> MDSTSTIANKIEEYLGAKSDDSKIDELLKADPSEVEYYRSGGDGDYLKNNICKITVNHSDSGKYDPCEKKLPPYDDNDQWKCQQNSSDGSGKPENICVPPRRERLCTYNLENLKFDKIRDNNAFLADVLLTARNEGEKIVQNHPDTNSSNVCNALERSFADLADIIRGTDQWKGTNSNLEKNLKQMFAKIRENDKVLQDKYPKDQKYTKLREAWWNANRQKVWEVITCGARSND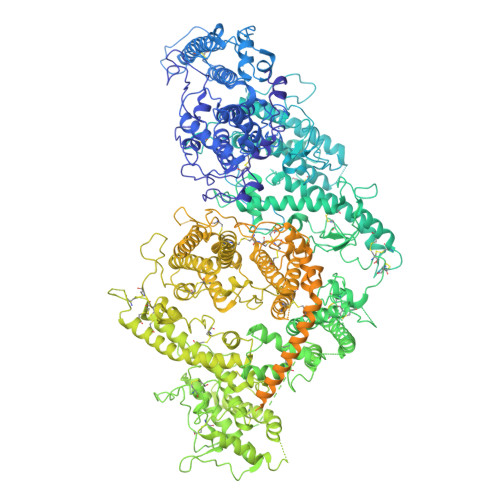LLIKRGWRTSGKSDRKKNFELCRKCGHYEKEVPTKLDYVPQFLRWLTEWIEDFYREKQNLIDDMERHREECTREDHKSKEGTSYCSTCKDKCKKYCECVKKWKTEWENQENKYKDLYEQNKNKTSQKNTSRYDDYVKDFFEKLEANYSSLENYIKGDPYFAEYATKLSFILNPSDANNPSGETANHNDEACNCNESGISSVGQAQTSGPSSNKTCITHSSIKTNKKKECKDVKLGVRENDKDLKICVIEDTSLSGVDNCCCQDLLGILQENCSDNKRGSSSNDSCDNKNQDECQKKLEKVFASLTNGYKCDKCKSGTSRSKKKWIWKKSSGNEEGLQEEYANTIGLPPRTQSLYLGNLPKLENVCEDVKDINFDTKEKFLAGCLIVSFHEGKNLKKRYPQNKNSGNKENLCKALEYSFADYGDLIKGTSIWDNEYTKDLELNLQNNFGKLFGKYIKKNNTAEQDTSYSSLDELRESWWNTNKKYIWTAMKHGAEMNITTCNADGSVTGSGSSCDDIPTIDLIPQYLRFLQEWVENFCEQRQAKVKDVITNCKSCKESGNKCKTECKTKCKDECEKYKKFIEACGTAGGGIGTAGSPWSKRWDQIYKRYSKHIEDAKRNRKAGTKNCGTSSTTNAAASTDENKCVQSDIDSFFKHLIDIGLTTPSSYLSNVLDDNICGADKAPWTTYTTYTTTEKCNKERDKSKSQSSDTLVVVNVPSPLGNTPYRYKYACQCKIPTNEETCDDRKEYMNQWSCGSARTMKRGYKNDNYELCKYNGVDVKPTTVRSNSSKLDGNDVTFFNLFEQWNKEIQYQIEQYMTNANISCIDEKEVLDSVSDEGTPKVRGGYEDGRNNNTDQGTNCKEKCKCYKLWIEKINDQWGKQKDNYNKFRSKQIYDANKGSQNKKVVSLSNFLFFSCWEEYIQKYFNGDWSKIKNIGSDTFEFLIKKCGNNSAHGEEIFSEKLKNAEKKCKENESTDTNINKSETSCDLNATNYIRGCQSKTYDGKIFPGKGGEKQWICKDTIIHGDTNGACIPPRTQNLCVGELWDKSYGGRSNIKNDTKELLKEKIKNAIHKETELLYEYHDTGTAIISKNDKKGQKGKNDPNGLPKGFCHAVQRSFIDYKNMILGTSVNIYEHIGKLQEDIKKIIEKGTPQQKDKIGGVGSSTENVNAWWKGIEREMWDAVRCAITKINKKNNNSIFNGDECGVSPPTGNDEDQSVSWFKEWGEQFCIERLRYEQNIREACTINGKNEKKCINSKSGQGDKIQGACKRKCEKYKKYISEKKQEWDKQKTKYENKYVGKSASDLLKENYPECISANFDFIFNDNIEYKTYYPYGDYSSICSCEQVKYYKYNNAEKKNNKSLCYEKDNDMTWSKKYIKKLENGRSLEGVYVPPRRQQLCLYELFPIIIKNEEGMEKAKEELLETLQIVAEREAYYLWKQYNPTGKGIDDANKKACCAIRGSFYDLEDIIKGNDLVHDEYTKYIDSKLNEIFGSSNTNDIDTKRARTDWWENETITNGTDRKTIRQLVWDAMQSGVRYAVEEKNENFPLCMGVEHIGIAKPQFIRWLEEWTNEFCEKYTKYFEDMKSKCDPPKRADTCGDNSNIECKKACANYTNWLNPKRIEWNGMSNYYNKIYRKSNKESEDGKDYSMIMAPTVIDYLNKRCHGEINGNYICCSCKNIGAYNTTSGTVNKKLQKKETECEEEKGPLDLMNEVLNKMDKKYSAHKMKCTEVYLEHVEEQLNEIDNAIKDYKLYPLDRCFDDQTKMKVCDLIADAIGCKDKTKLDELDEWNDMDLRGTYNKHKGVLIPPRRRQLCFSRIVRGPANLRSLNEFKEEILKGAQSEGKFLGNYYKEHKDKEKALEAMKNSFYDYEDIIKGTDMLTNIEFKDIKIKLDRLLEKETNNTKKAEDWWKTNKKSIWNAMLCGYKKSGNKIIDPSWCTIPTTETPPQFLRWIKEWGTNVCIQKQEHKEYVKSKCSNVTNLGAQASESNNCTSEIKKYQEWSRKRSIQWETISKRYKKYKRMDILKDVKEPDANTYLREHCSKCPCGFNDMEEMNNNEDNEKEAFKQIKEQVKIPAELEDVIYRIKHHEYDKGNDYICNKYKNIHDRMKKNNGNFVTDNFVKKSWEISNGVLIPPRRKNLFLYIDPSKICEYKKDPKLFKDFIYWSAFTEVERLKKAYGGARAKVVHAMKYSFTDIGSIIKGDDMMEKNSSDKIGKILGDTDGQNEKRKKWWDMNKYHIWESMLCGYREAEGDTETNENCRFPDIESVPQFLRWFQEWSENFCDRRQKLYDKLNSECISAECTNGSVDNSKCTHACVNYKNYILTKKTEYEIQTNKYDNEFKNKNSNDKDAPDYLKEKCNDNKCECLNKHIDDKNKTWKNPYETLEDTFKSKCDCPKPLPSPIKPDDLPPQADEPF>[4x]MRIPLV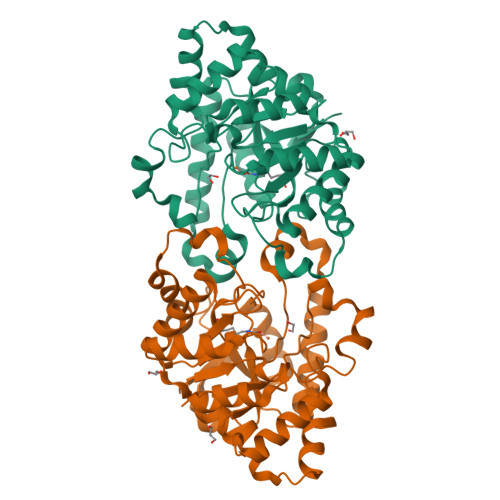GKDSIESKDIGFTLIHEHLRVFSEAVRQQWPHLYNEDEELRNAVNEVKRAMQFGVKTIVDPTVMGLGRDIRFMEKVVKATGINLVAGTGIYIYIDLPFYFLNRSIDEIADLFIHDIKEGIQGTLNKAGFVKIAADEPGITKDVEKVIRAAAIANKETKVPIITHSNAHNNTGLEQQRILTEEGVDPGKILIGHLGDTDNIDYIKKIADKGSFIGLDRYGLDLFLPVDKRNETTLRLIKDGYSDKIMISHDYACTIDMGTAKPEYKPKLAPRWSTTLIFEDTIPFLKRNGVNEEVIATIFKENPKKFFS pmcThe BEN (BANP, E5R, and NAC1) domain is a ∼100-residue protein domain found in metazoans and viruses, but missing in nematodes and urochordates. There are nine BEN domain–containing transcription factors in the human genome, i.e., BANP, BEND2-7, and NAC1/2. The BEN domain-containing transcription factors regulate transcription by recruiting chromatin-modifying factors to specific chromatin regions via their DNA-binding BEN domains. Further structural analysis revealed that although all these BEN domains bind their target DNAs mainly through the insertion of the C-terminal α5 helix into the major groove of DNA, the residues of the α5 helices involved in the base interactions vary from one to another, explaining why they exhibit distinct DNA sequence preference.

BANP has been reported to prefer unmethylated DNA, and methylation in the CGCG motif significantly reduces its binding affinity to BANP. Our ITC results showed that the mCGCG DNA displayed only a 2-fold weaker binding affinity to the BANP BEN domain than the unmethylated CGCG DNA, and the CGmCG DNA exhibited a similar binding affinity to the unmethylated CGCG DNA. Hence, our binding assay results indicated that the BANP BEN domain was likely a methylation-insensitive DNA binder. To illustrate the molecular mechanism of the BANP BEN domain in recognizing the methylated DNA, we obtained the crystal structure of the BANP BEN domain bound to an mCGCG DNA. Similarly, the C-terminal region after the helix α5 is disordered in the BANP-mCGCG structure. Superposition of the structures of the BANP-CGCG and BANP-mCGCG complexes revealed that these two structures superimposed well with an RMSD of 0.34 Å over their 104 Cα atoms, suggesting that the methylation of the cytosine within the DNA did not cause significant conformational changes. Like the BANP-CGCG structure, the BANP BEN domain interacted with the methylated DNA mainly through its α5 helix. Similarly, in the BANP-mCGCG complex, the side chain of S313 formed a hydrogen bond with the base of T4, and the side chain of R316 formed two hydrogen bonds with the base of G5′ that is complementary with the methylcytosine, while the methyl group of mC was not involved in the BANP binding. In addition to the base interactions, Loop 1 also was involved in the interactions with the backbone of DNA via the residues N269, S271, H276, and K278.

>GNSEEDYPNGTWLGDENNPEMRVRCAIIPSDMLHISTNCRTAEKMALTLLDYLFHREVQAVSNLSGQGKHGKKQLDPLTIYGIRCHLFYKFGITESDWYRIKQSIDSKCRTAWRRKQRGQSLAVKSFSRRTPNSSSYCPSE[2x]> MQKRQSTKEEVYKDFQKQISDMNYYSCKAEVEVVGNKSPHNYVLIHTYKKTDNYKLEVISPKHLKGKSIEYQGDKILVKNPKISDVVELPNTGKNNQYLFVGDFIKNYLQNEEMKVKLSKGHLVLETFIPGDNKYFNKQVLYVNADTKNPEKMEVLDKEGVPRFTVKYKDFEYRN;> MKNISEDVIKYMPVTNKTIILDAGHGGIDPGALNKDKSTSEKDINLAITLKLRELIESSGGLVILTREDDSSLYKEENNKTTRQKYNENLKNRKEIISNSNANMFVSIHLNAFEQSKYYGAQTFYPKDKQDSKELSKCIQEELKRVVDKTNNREVKPRDDIYLLKDNNIPSVLIECGFLSNEKECKLLTDETYQEKIAWAIYIGIQKYLSVDKLAAA

In C. difficile, MAL production depends on the CwlD amidase and its binding partner, the GerS lipoprotein. CwlD removes the peptide side chain from N-acetylmuramic acid (NAM) so that PdaA can deacetylate NAM and catalyze lactam ring formation to form MAL. Amidase_3 family members are Zn2+-dependent N-acetylmuramoyl amidases that use a Zn2+ ion as part of their catalytic mechanism. While the functions of CwlD and PdaA are conserved between B. subtilis and C. difficile, we recently showed that C. difficile CwlD amidase activity depends on the GerS lipoprotein.

The asymmetric unit contained one molecule of CwlD and one monomer of GerS with the CwlD structure being typical of the amidase superfamily. GerS is largely anti-parallel beta sheet with the exception of an N-terminal alpha helix and forms a cupped hand-like shape similar to the LolA family of lipid-associated proteins. While the members of the LolA family are typically monomeric, completion of the beta fold for GerS required two molecules such that the N-terminal alpha helix through the first 2 beta strands comes from one molecule in the crystal and the remainder of the GerS fold comes from a symmetry mate. Thus, the likely biological assembly for the CwlD:GerS complex contains two molecules of GerS and two CwlD and is in agreement with both dynamic light scattering (DLS) data and size exclusion chromatography. The structure of CwlD is the mixed alpha-beta fold expected for the N-acetylmuramoyl-L-alanine amidase superfamily, with 3 conserved glutamate residues and 2 histidines coordinating the Zn2+ ion. His49 (positioned by Glu53), His133, and the carboxylate of Glu65 provide four of the ligands of the near octahedral ion coordination with distances of 2.2 Å. While CwlD does not have an autoinhibitory helix, the N-terminus of a GerS symmetry molecule provides the additional liganding for the Zn2+. As this symmetry molecule is not one from the 2 GerS monomers used to bind CwlD, the interaction is not physiologically relevant. Importantly, the binding orientation for CwlD relative to GerS leaves the CwlD Zn2+-containing active site solvent accessible to substrate rather than at the complex interface. Alpha helix 1 (residues 65–82) and the C-terminal alpha helix (residues 217–235) of CwlD constitute the most significant interface with GerS contacting stands 2 through 6.>[2x]MKRVLVTLGAVAALATGAVAGGGAHWGYSGSIGPEHWGDLSPEYLMCKIGKNQSPIDINSADAVKACLAPVSVYYVSDAKYVVNNGHTIKVVMGGRGY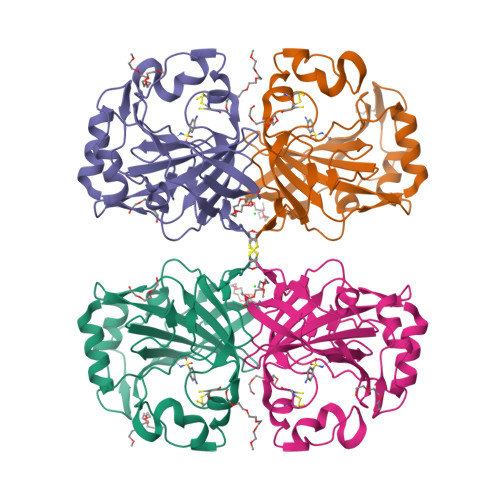VVVDGKRFYLKQFHFHAPSEHTVNGKHYPFEAHFVHLDKNGNITVLGVFFKVGKENPELEKVWRVMPEEPGQKRHLTARIDPEKLLPENRDYYRYSGSLTTPPCSEGVRWIVFKEPVEMSREQLEKFRKVMGFDNNRPVQPLNARKVMK>GMASRSRRPERRQEPLSRERIVGAAVELLDTVGERGLTFRALAERLATGPGAIYWHITGKAELLGAATDAVVTAAVTAGPTGAADSPQDAVRAVALGLWDATEAHPWLATQLATQLSRTPWGTVAPRIFESLGRQVQAMGVPEAHWFTASSALMHYILGAAGQNAANSASAGPVGADVDRDEFLDTVSTAWEGLDPDAYPFTRAVADQVRGHDDREQFLAGITLVLTGITALHRPGR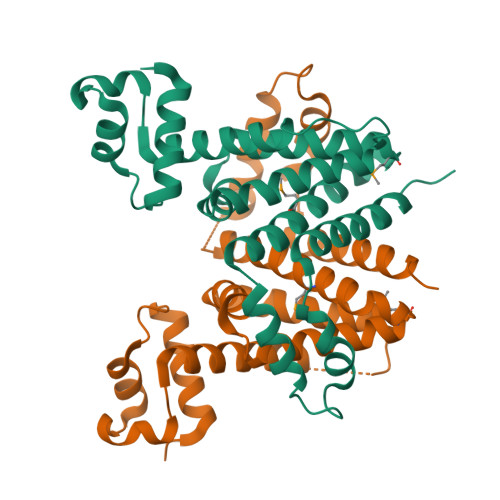[2x]> GSASTVKGSVDLEKLAFGLTKLNEDDLVGVVQMVTDNKTPEMNVTNNVE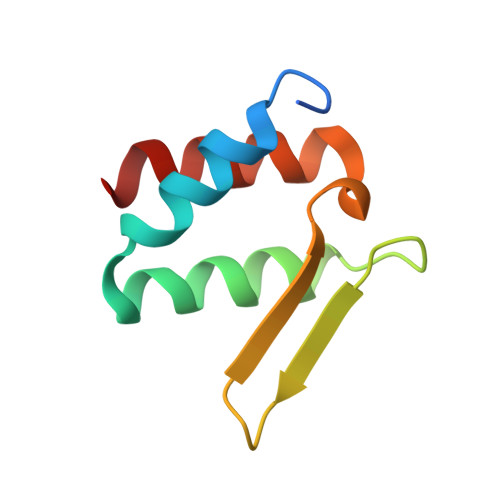EGEFIIDLYSLPEGLLKSLWDYVKKNT>[2x]ESTSLYKKAGLKPQVYHVDAFTSQPFRGNSAGVVFPADNLSEAQMQLIARELGHSETAFLLHSDDSDVRIRYFTPTVEVPICGHATVAAHYV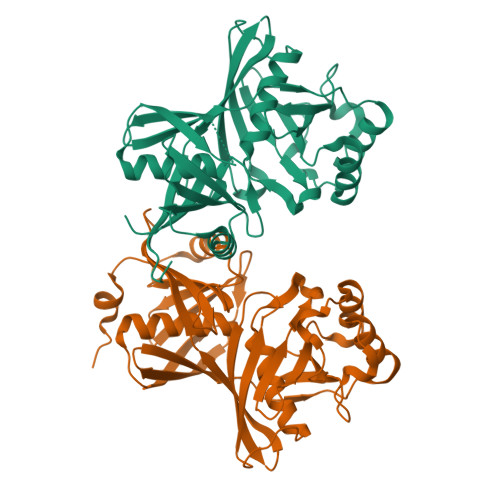RAKVLGLGNCTIWQTSLAGKHRVTIEKHNDDYRISLEQGTPGFEPPLEGETRAAIINALHLTEDDILPGLPIQVATTGHSKVMIPLKPEVDIDALSPDLNALTAISKKIGCNGFFPFQIRPGKNETDGRMFSPAIGIVEDPVTGNANGPMGAWLVHHNVLPHDGNVLRVKGHQGRALGRDGMIEVTVTIRDNQPEKVTISGTAVILFHAEWAIEL>SMTEIRVHQGDLPNLDNYRIDAVAVDTETLGLQPHRDRLCVVQLSSGDGTADVIQIAKGQKSAPNLVRLLSDRDITKIFHFGRFDLAILAHTFGVMPDVVFCTKIASKLTRTYTDRHGLKEICGELLNVN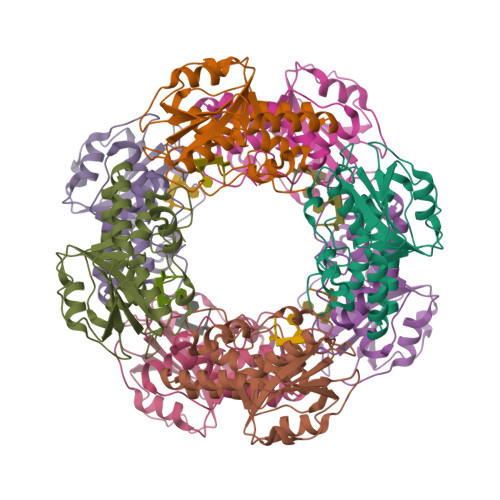ISKQQQSSDWAAETLSRAQIEYAASDVLYLHRLKDIFEERLKREERESVAKACFQFLPMRANLDLLGWSEIDIFAHS[8x]>GPLGSSMEDHDDHLRRKFMEFPYVSPTRKQLMVDLMSTVENRLQSQLLPCNLPPDVRNFNNPNGSAEASLHIRSGDKSSPIDFVIGSWIHCKIPTGVSLNITSISGFLNSSTKAPNFVVELIQSSSKSLVLILDLPHRKDLVLNPDYLKEYYQDTALDSHRQSLLKLPEVNPYVSPSLFVRSAFSPTASMLKIDAEEEDKLEEILRDHVSPAAKEVLEVWLERCVKEEEEKIVVGEEERMELERRDKSFRRKSIEDDLDL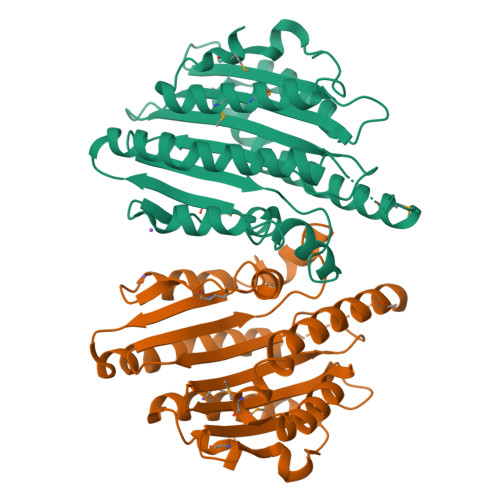QFPRMFGEEVSSRVVHAIKEAFGVL[2x]>GMEMTKVTGKFDVKLTPENAYATGVGGVNLGRMALDKTFYGELEARSQGEMLSA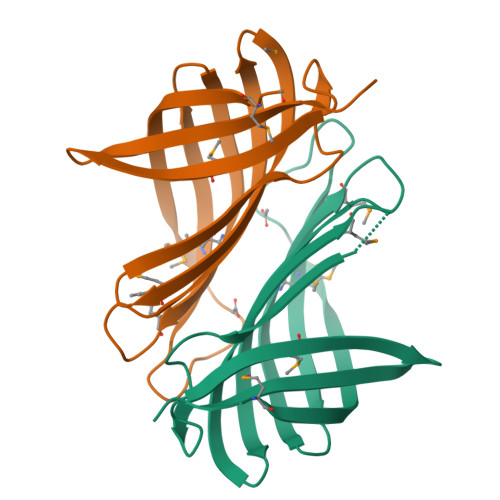MTAVKGSAGYVAIEQVVGKLCGRQGSFVLQHFGIMTDGQNRLHLEVVPHSGAGELTGLYGTMAISIENGQHFYEFSFCFEPASEVEG[2x]> KVEQAVETEPEPELRQQTEWQSGQRWELALGRFWDYLRWVQTLSEQVQEELLSSQVTQELRALMDETMKELKAYKSELEEQLTPVAEETRARLSKELQAAQARLGADMEDVCGRLVQYRGEVQAMLGQSTE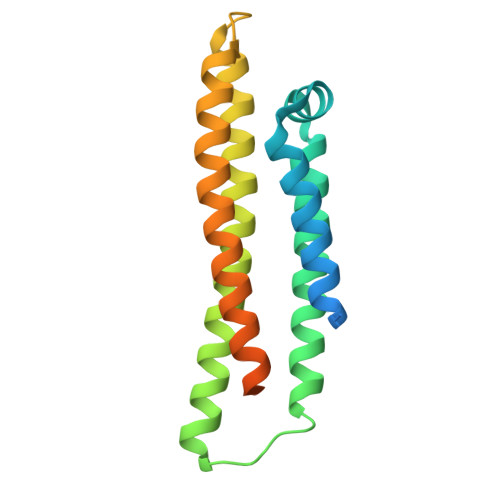ELRVRLASHLRKLRQRLLRDADDLQKRLAVYQAGAREGAERGLSAIRERLGPLVEQGRVR> GSESSRSAMMYIQELRSGLRDMHLLSCLESLRVSLNNNPVSWVQTFGAEGLASLLDILKRLHDEKEETSGNYDSRNQHEIIRCLKAFMNNKFGIKTMLETEEGILLLVRAMDPAVPNMMIDAAKLLSALCILPQPEDMNERVLEAMTERAEMDEVERFQPLLDGLKSGTSIALKV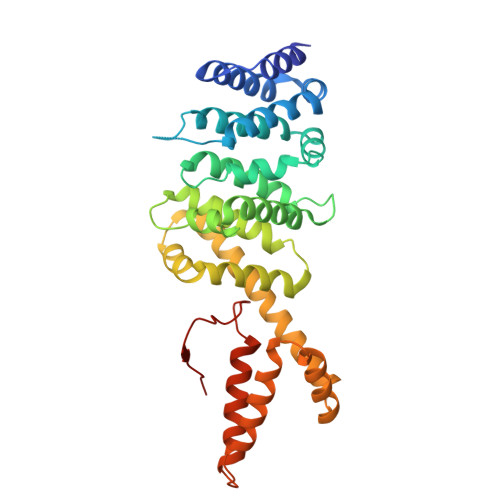GCLQLINALITPAEELDFRVHIRSELMRLGLHQVLQELREIENEDMKVQLCVFDEQGDEDFFDLKGRLDDIRMEMDDFGEVFQIILNTVKDSKAEPHFLSILQHLLLVRNDYEARPQYYKLIEECVSQIVLHKNGTDPDFKCRHLQIDIERLVDQ> MRGWHHHHHHGIRMRARYPSVVDVYSVEQFRNIM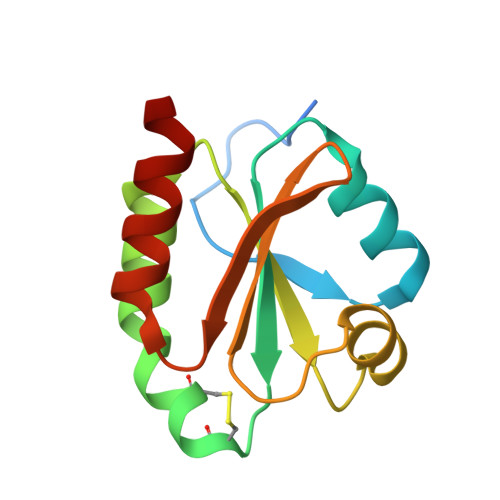SEDILTVAWFTAVWCGPCKTIERPMEKIAYEFPTVKFAKVDADNNSEIVSKCRVLQLPTFIIARSGKMLGHVIGANPGMLRQKLRDIIKDN> GHMGQKASQQLALKDSKEVPVVCEVVSEAIVHAAQKLKEYLGFEYPPSKLCPAANTLNEIFLIHFITFCQEKGVDEWLTTTKMTKHQAFLFGADWIWTFWGSDKQIKLQLAVQTLQMSSPPPVESKPCDLSNPESRV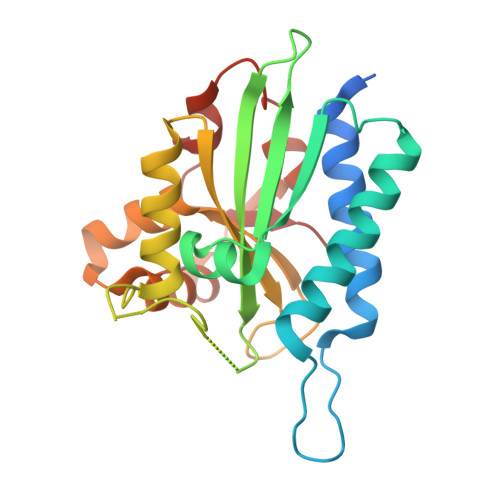EESSWKKSRFDKLEEFCNLIGEDCLGLFIIFGMPGKPKDIRGVVLDSVKSQMVRSHLPGGKAVAQFVLETEDCVFIKELLRNCLSKKDGLREVGKVYISIL> MALNKVQLIKLYSNRLVKSLVPVEFGEAFIQSIINDLQTTLLNTSSEEQNLSIIINKLKMQFLSNNLKNEWVEFQNIVNSLSKFKSLDQICNYLAFLDALRDEKPEDILSTSTASLSPGKQNLMINTVNTALTLSQLIEPYYDTLSEQTILTYLPYTMLGSDSKIFTFSNNYTRLEIPKDINNSFSSLLREVFEF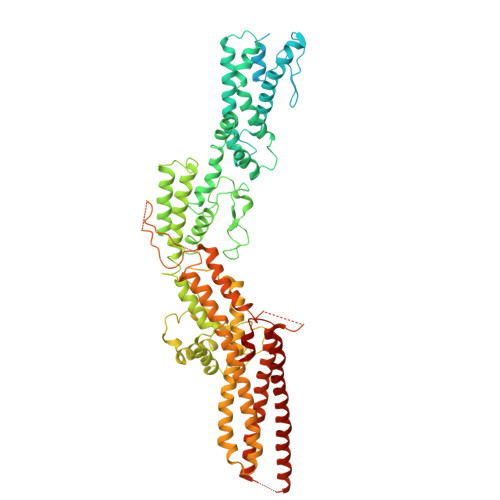AILYKQLAIVVDRYKGTLVSAIKTAYIAILEAQLNKYVNDINNIFNNKPNSILVVYNSIFPWISILRFLYRVSNRLNRLDGYEFLTFIYSFTNHGDPKIRGIAVTAFTEVVKPYYNIVEHWIVKGELIDNNNEFFIIFDQEQNEFNSIIKLLPKKIPAFIKSSDKIFQIGKTLIFLNKYCRELKWVNQYNVKYSAILFNNHQGLASMTTNEMIKLIDSQYNEILTFLTQIIQGNNKLFTHVYNFKRFYFMETNDFIDAIMVKGKDVFNESSVNISSTYLRKVLQDAIQISSVKNFEYVDRLDSRVLNPQHGNLGWESFTIEYKIDDLPMSYLFEGHQHLQYLKMFHFLWKLRQLNNLLNWHFEMFNELNHNVVTKLSSRNRRPLAKSLSIITSIRFHFTQFLNELIAYLSYDVIEENFQQHIVRKLFYNKNDQDLLLNKSFMNLSEIDPNNDLPKFNVNLLTIDELVELHGTYIDSIINSSLLNEKLKGNETNISYIDQIFNILQTIFNFINTSQEFYSLVVTFGLLVRSDSNANKIELEQDQEDLEFQLHKIKRKIYKDIYQHDYKRQLNDLKNDLNRDYNLKDLSKLL> NLQNIIYNPVIPFVGTIPDQLDPGTLIVIRGHVPSDADRFQVDLQNGSSMKPRADVAFHFNPRFKRAGCIVCNTLINEKWGREEITYDTPFKREKSFEIVIMVLKDKFQVAVNGKHTLLYGHRIGPEKIDTLGIYGKVNIHSIGFSFSSD;> NNLQNIIYNPVIPFVGTIPDQLDPGTLIVIRGHVPSDADRFQVDLQNGSSMKPRADVAFHFNPRFKRAGCIVCNTLINEKWGREEITYDTPFKREKSFEIVIMVLKDKFQVAVNGKHTLLYGHRIGPEKIDTLGIYGKVNIHSIGFSFSSD

pmcGalectins are a family of proteins that bind β-d-galactopyranoside-containing glycoconjugates through their canonical carbohydrate recognition domains (CRDs). Galectin-8 is a divalent galectin found in the liver, the kidney, the cardiac muscle, the lung, and the brain. Galectin-8 is a carbohydrate-binding protein that plays a crucial role in tumor progression and metastasis, antibacterial autophagy, modulation of the immune system, and bone remodeling. However, there are major differences between the two CRDs, such as the presence of Arg45, Arg59, Tyr141, and Gln47 in the N-terminal CRD (galectin-8N) and the presence of Ser255, Asn257, and Asn348 in the C-terminal CRD (galectin-8C).

Galectin-8N was first cocrystallized with lactose, and then the ligands were soaked into galectin-8N-lactose crystals, followed by collection of X-ray diffraction data at 1.52 and 2.1 Å resolution for the galectin-8N–6a complex and galectin-8N–9 complex, respectively. Both complexes showed that the O4 and O6 of the d-galactal portion bind to galectin-8N in a similar manner as the corresponding oxygens in the d-galactosides. Namely, the O4 of the d-galactal is involved in a hydrogen-bonding network with Arg45, Arg69, and His65. Further, the O6 of the d-galactal engages in hydrogen bonding interactions with Asn79 and Glu89, while the O3 engages in a hydrogen bonding interaction with Arg45. As for the galectin-8N–9 complex, the quinoline ring is placed in a favorable position to establish an interaction with Arg45 while the carboxylate moiety establishes a water-mediated hydrogen bond with Gln47 and Arg45. The endocyclic double bond of the d-galactal moiety in both complexes is placed in proximity to the guanidinium side chains of Arg45 and Arg69. Compounds 6a, 6c, and 9 had nearly identical Kd values for galectin-8N, with compound 6c exhibiting the highest gain in binding affinity compared to its galactoside equivalent with a Kd of 46 μM.>MAAGVAAWLPFARAAAIGWMPVASGPMPAPPRQERKRTQDALIVLNVSGTRFQTWQDTLERYPDTLLGSSERDFFYHPETQQYFFDRDP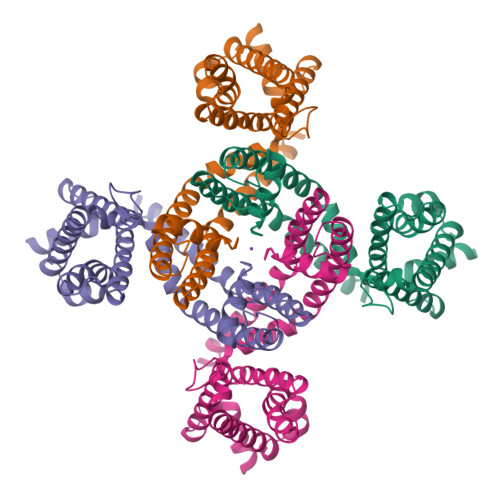DIFRHILNFYRTGKLHYPRHECISAYDEELAFFGLIPEIIGDCCYEEYKDRRRENAERLQDDADTDTAGESALPTMTARQRVWRAFENPHTSTMALVFYYVTGFFIAVSVIANVVETVPCGSSPGHIKELPCGERYAVAFFCLDTACVMIFTVEYLLRLAAAPSRYRFVRSVMSIIDVVAILPYYIGLVMTDNEDVSGAFVTLRVFRVFRIFKFSRHSQGLRILGYTLKSCASELGFLLFSLTMAIIIFATVMFYAEKGSSASKFTSIPAAFWYTIVTMTTLGYGDMVPKTIAGKIFGSICSLSGVLVIALPVPVIVSNFSRIYHQNQRADKRRAQKKARLARIRAAKSGSANAYMQSKRNGLLSNQLQSSEDEQAFVSKSGSSFETQHHHLLHCLEKTTNHEFVDEQVFEESCMEVATVNRPSSHSPSLSSQQGVTSTCCSRRHKKTFRIPNANVSGSHQGSIQELSTIQIRCVERTPLSNSRSSLNAKMEECVKLNCEQPYVTTAIISIPTPPVTTPEGDDRPESPEYSGGNIVRVSAL[4x]> YNLDVRGARSFSPPRAGRHFGYRVLQVGNGVIVGAPGEGNSTGSLYQCQSGTGHCLPVTLRGSNYTSKYLGMTLATDPTDGSILACDPGLSRTCDQNTYLSGLCYLFRQNLQGPMLQGRPGFQECIKGNVDLVFLFDGSMSLQPDEFQKILDFMKDVMKKLSNTSYQFAAVQFSTSYKTEFDFSDYVKWKDPDALLKHVKHMLLLTNTFGAINYVATEVFREELGARPDATKVLIIITDGEATDSGNIDAAKDIIRYIIGIGKHFQTKESQETLHKFASKPASEFVKILDTFEKLKDLFTELQKKIYVIEGTSKQDLTSFNMELSSSGISADLSRGHAVVGAVGAKDWAGGFLDLKADLQDDTFIGNEPLTPEVRAGYLGYTVTWLPSRQKTSLLASGAPRYQHMGRVLLFQEPQGGGHWSQVQTIHGTQIGSYFGGELCGVDVDQDGETELLLIGAPLFYGEQRGGRVFIYQRRQLGFEEVSELQGDPGYPLGRFGEAITALTDINGDGLVDVAVGAPLEEQGAVYIFNGRHGGLSPQPSQRIEGTQVLSGIQWFGRSIHGVKDLEGDGLADVAVGAESQMIVLSSRPVVDMVTLMSFSPAEIPVHEVECSYSTSNKMKEGVNITICFQIKSLIPQFQGRLVARLTYTLQLDGHRTRRRGLFPGGRHELRRNIAVTTSMSCTDFSFHFPVCVQDLISPIRVSLNFSLWEEEGTPRDQRAQGKDIPPILRPSLHSETWEIPFEKNPAALQTLFQGPLGAQGEKELQALEKENAQLEWELQALEKELAQHHH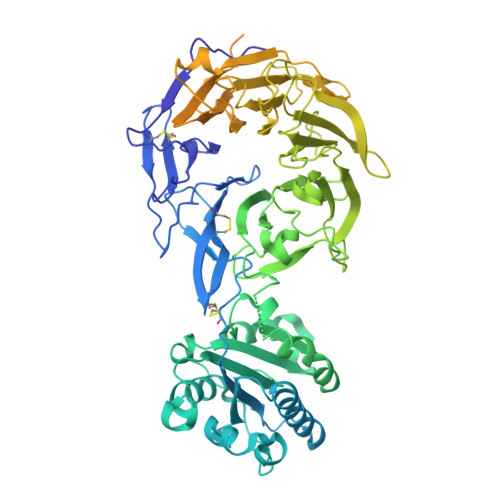HHHA>MIHLYDAKSFAKLRAAQYAAFHTDAPGSWFDHTSGVLESVEDGTPV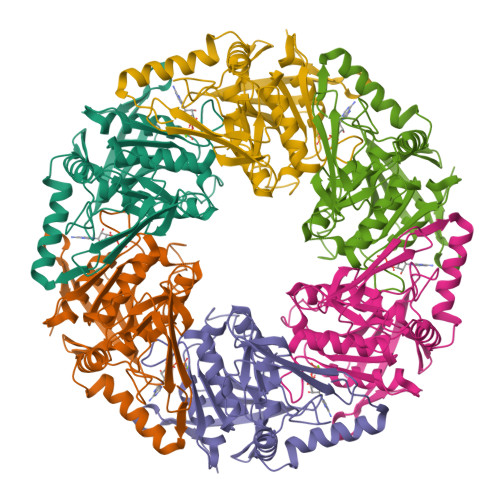LAIGVESGDAIVFDKNAQRIVAYKEKSVKAEDGSVSVVQVENGFMKQGHRGWLVDLTGELVGCSPVVAEFGGHRYASGMVIVTGKGNSGKTPLVHALGEALGGKDKYATVRFGEPLSGYNTDFNVFVDDIARAMLQHRVIVIDSLKNVIGAAGGNTTSGGISRGAFDLLSDIGAMAASRGCVVIASLNPTSNDDCIVELVKEASRSNSTSLVISTDVDGEWQVLTRTGEGLQRLTHTLQTSYGEHSVLTIHTSKQSGGKQASGKAIQTVIKNDELESVLRRLTSN[3x]> MSIDSALNWDGEMTVTRFDRMTGAHFVIRLDSTQLGPAAGGTRAAQYSQLADALTDAGKLAGAMTLKMAVSNLPMGGGKSVIALPAPRHSIDPSTWARILRIHAENIDKLSGNYWTGPDVNTNSADMDTLNDTTEFVFGRSLERGGAGSSAFTTAVGVFEAMKATVAHRGLGSLDGLTVLVQGLGAVGGSLASLAAEAGAQLLVADTDTERVAHAVALGHTAVALEDVLSTPCDVFAPCAMGGVITTEVARTLDCSVVAGAANNVIADEAASDILHARGILYAPDFVANAGGAIHLVGREVLGWSESVVHERAVAIGDTLNQVFEISDNDGVTPDEAARTLAGRRARE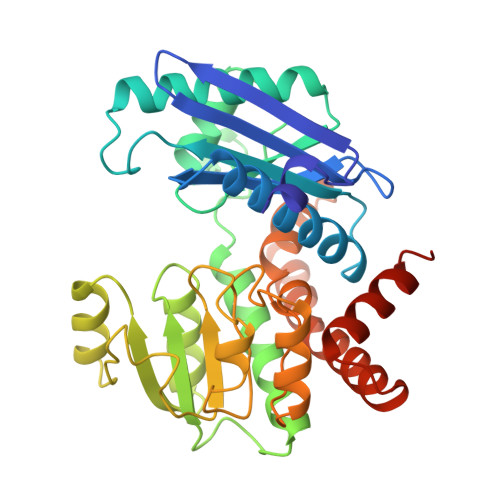ASTTTATA>PKFKFKFKFKFKP[1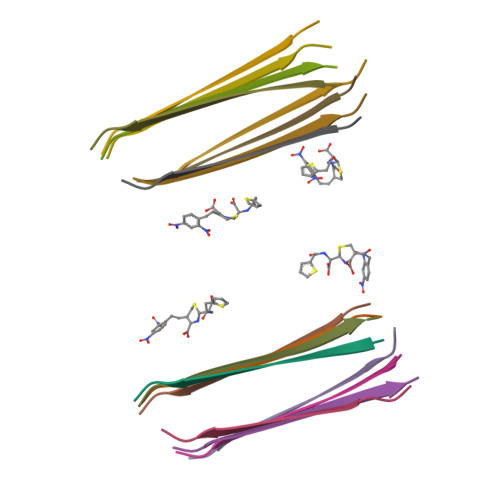6x]>MASWSHPQFEKSGGGGGLVPRGSQVFLEERLDGATGSSIVVTMEGTRPILAEVQALVTPTMFGNAKRTTTGLDFNRASLIMAVLEKRAGLLLQNQDAYLKSAGGVKLDEPAIDLAVAVAIASSYKDKPTNPQECFVGELGLTGEIRRVNRIEQRINEAAKLGFTKIYVPKNSLTGITLPKEIQVIGVTTIQEVLKKVF[2x]

We report here a detailed structural and functional analysis of the RadA protein from S. pneumoniae, which uncovers several key properties of this HR effector encoded in nearly all bacterial species and in some eukaryotes. All bacterial RadA proteins are characterized at the sequence level by three conserved domains: a potential C4-type zinc binding motif (C4); a central canonical RecA-like ATPase domain (H), including a KNRFG motif unique to and strictly conserved in RadA proteins; and a region homologous to the protease domain (P) of the bacterial Lon protein. In addition, like DnaB proteins, we show that RadA assembles into a ring-shaped hexamer and is a functional DNA helicase that loads onto ssDNA and translocates in a 3′ direction along it to unwind dsDNA. The full-length protein (RadAFL) and the P domain (RadAP) of pneumococcal RadA were purified from E. coli and shown to assemble predominantly as hexamers in solution.

The crystal structure of RadAP was solved at 2.5 Å resolution and the structure of RadAFL bound to thymidine diphosphate (dTDP) was solved at 3.5 Å resolution. In the structures of RadAP and RadAFL, the P domain (residues 290–453) forms a ring with six-fold symmetry. RadAP is structurally related to the proteolytic domain of Lon proteases (LonP), which also assembles into a stable annular hexamer, within the full-length protein and as an independent domain. However, the typical lysine and serine residues of the protease catalytic dyad in LonP are replaced in the pneumococcal RadAP domain by an arginine and an alanine, respectively. Furthermore, even though the sequence and the fold are similar, the electrostatic potentials of the inner side of the rings have opposite charges, namely negative in the LonP and positive in RadAP. Thus, RadAP appears to be structurally but not functionally related to LonP, both adopting the same ring-shaped hexameric architecture. In both RadAFL and RadAp, the hexameric structure is primarily maintained by the extensive surface of interaction between adjacent P domains (940–976 Å). The structure of pneumococcal RadA shows that its P domain forms a stable scaffold to assemble the helicase central motor in the full-length hexamer. The internal diameter of the P domain (15 Å) can accommodate ssDNA but not dsDNA. In addition, the stability provided by the robust self-association of RadA P domain into a hexameric ring allows RadA to promote incorporation into the genome of transforming ssDNA over long distances.> MEPPVQVAVIGSGGAAMAAALKAVEQGAQVTL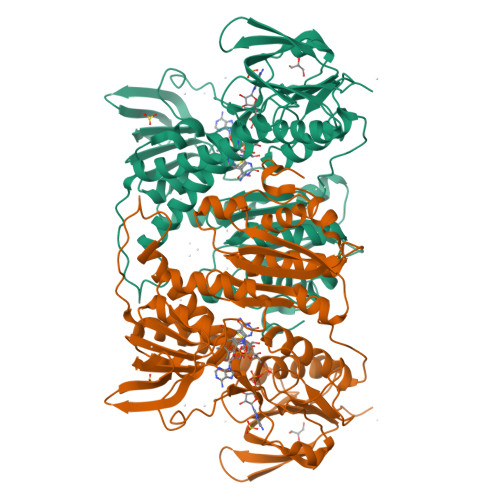IERGTIGGTCVNVGCVPSKIMIRAAHIAHLRRESPFDGGIAATVPTIDRSKLLAQQQARVDELRHAKYEGILGGNPAITVVHGEARFKDDQSLTVRLNEGGERVVMFDRCLVATGASPAVPPIPGLKESPYWTSTEALASDTIPERLAVIGSSVVALELAQAFARLGSKVTVLARNTLFFREDPAIGEAVTAAFRAEGIEVLEHTQASQVAHMDGEFVLTTTHGELRADKLLVATGRTPNTRSLALDAAGVTVNAQGAIVIDQGMRTSNPNIYAAGDCTDQPQFVYVAAAAGTRAAINMTGGDAALDLTAMPAVVFTDPQVATVGYSEAEAHHDGIETDSRTLTLDNVPRALANFDTRGFIKLVIEEGSHRLIGVQAVAPEAGELIQTAALAIRNRMTVQELADQLFPYLTMVEGLKLAAQTFNKDVKQLSAAAG> MGGRALRVLVDMDGVLADVEGGLLRKFRARFPDQPFIALEDRRGYKACEQYGRLRPGLSEKARSIAESKNFFFELEPLPGAVEAVKEMASLQNTDVFICTSPHKMFKYCPYEKYAWVEKYFGPDFLEQIVLTRDKTV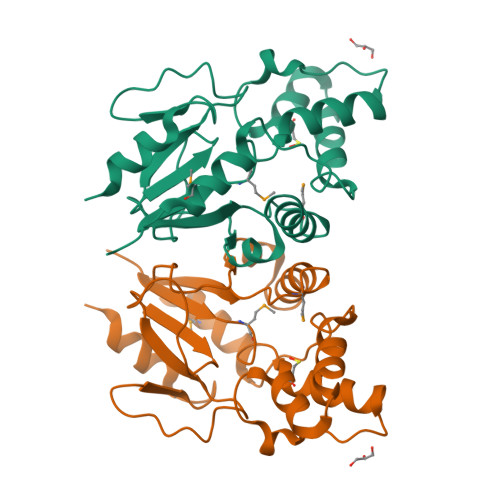VSADLLIDDRPDITGAEPTPSWEHVLFTACHNQHLQLQPPRRRLHSWADDWKAILDSKRPCGSLEHHHHHH>[2x]MGHHHHHHMSDDEHHFEASESGASKTYPQSAGNIRKGGHIVIKNRPCKVVEVSTSKTGK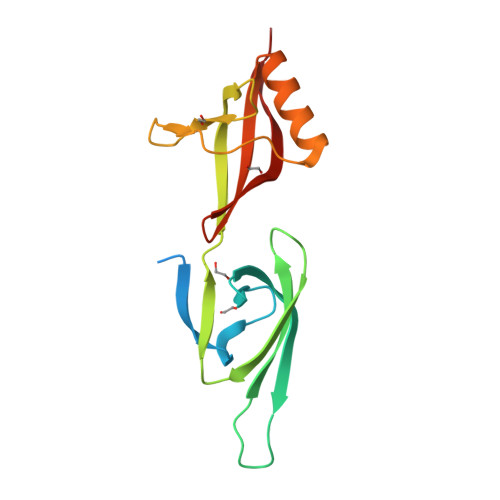HGHAKCHFVAIDIFTAKKLEDIVPSSHNCDVPHVNRVDYQLIDITEDGFVSLLTDSGGTKDDLKLPTDDGLTAQMRLGFDEGKDIVVSVMSSMGEEQICAVKEVGGGK> GSMGPRNDKIKHVQNQVDEVIDVMQENITKVIERGERLDELQDKSESLSDNATAFSNRSKQLRRQMWWR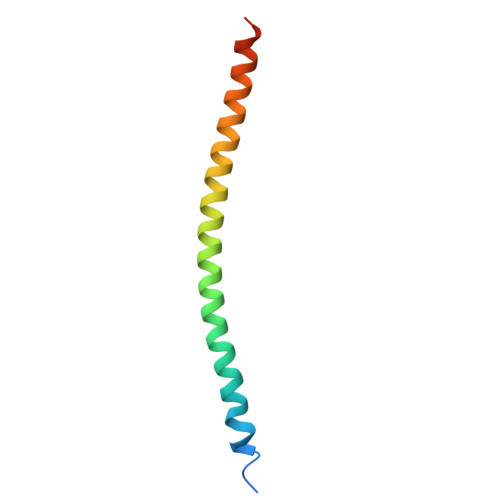GCKIK(5-methoxy-2-{[(4-methoxyphenyl)sulfonyl]carbamoyl}-1H-indol-1-yl)acetic 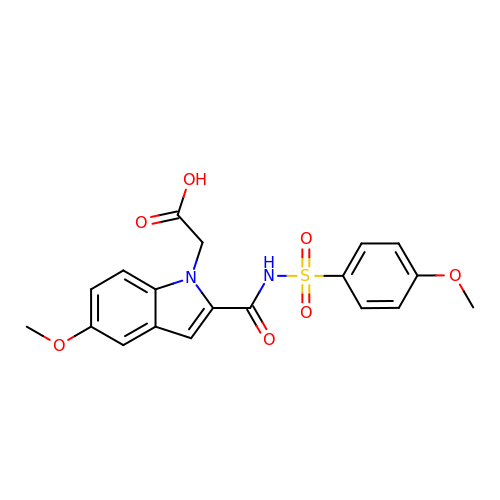acid | C19 H18 N2 O7 S | RSBKMGDPRRZEJA-UHFFFAOYSA-N> MFARLIRYFQEARAELARVTWPTREQVVEGTQAILLFTLAFMVILGLYDTVFRFLIGLLR;> MDLLYTLVILFYLGVAGLLVYLVLVQEPKQGAGDLMGGSADLFSARGVTGGLYRLTVILGVVFAALALVIGLWPR;> MVKAFWSALQIPELRQRVLFTLLVLAAYRLGAFIPTPGVDLDKIQEFLRTAQGGVFGIINLFSGGNFERFSIFALGIMPYITAAIIMQILVTVVPALEKLSKEGEEGRRIINQYTRIGGIALGAFQGFFLATAFLGAEGGRFLLPGWSPGPFFWFVVVVTQVAGIALLLWMAERITEYGIGNGTSLIIFAGIVVEWLPQ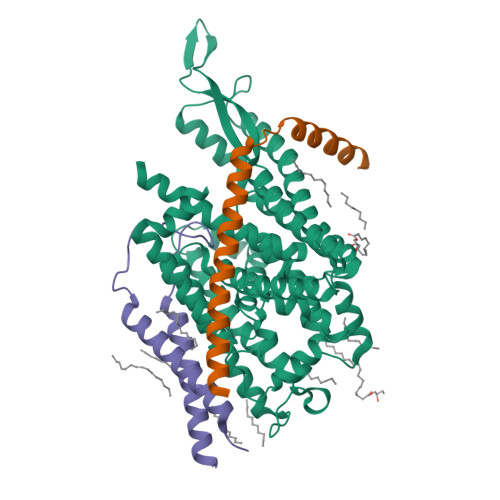ILRTIGLIRTGEVNLVAFLFFLAFIVLAFAGMAAVQQAERRIPVQYARKVVGGRVYGGQATYIPIKLNAAGVIPIIFAAAILQIPIFLAAPFQDNPVLQGIANFFNPTRPSGLFIEVLLVILFTYVYTAVQFDPKRIAESLREYGGFIPGIRPGEPTVKFLEHIVSRLTLWGALFLGLVTLLPQIIQNLTGIHSIAFSGIGLLIVVGVALDTLRQVESQLMLRSYEGFLSRGRLRGRNRHHHHHH>[6x]MGGSHHHHHHGMASGSPPTQPSPASDSGSGYVPGSVSAAFVTCPNEKVAKEIARAVVEKRLAACVNLIPQI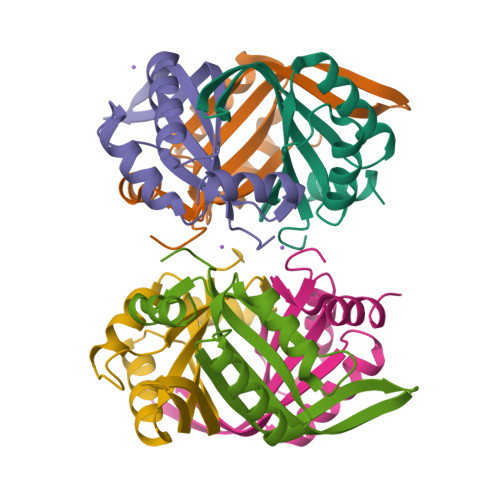TSIYEWKGKIEEDSEVLMMIKTQSSLVPALTDFVRSVHPYEVAEVIALPVEQGNFPYLQWVRQVTESVSDSITVLP>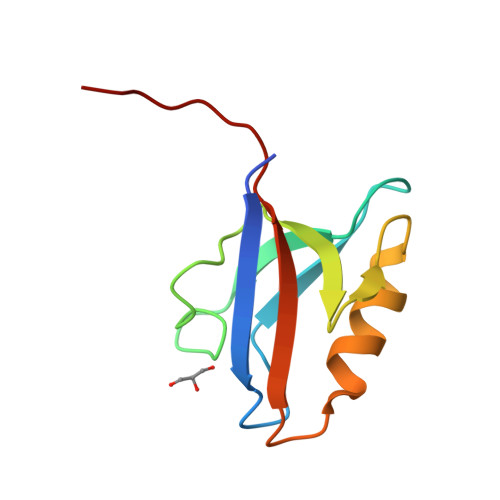 GPKGTEKTVKVIKDGPALGLTISDNGAGYAFIKKIREDSIMSRVANVAVGDHIAKINGTDLNGCRHFEVARMLKEIPIGSEFTMICVEPKKSFDEI> YGGGSSGGGS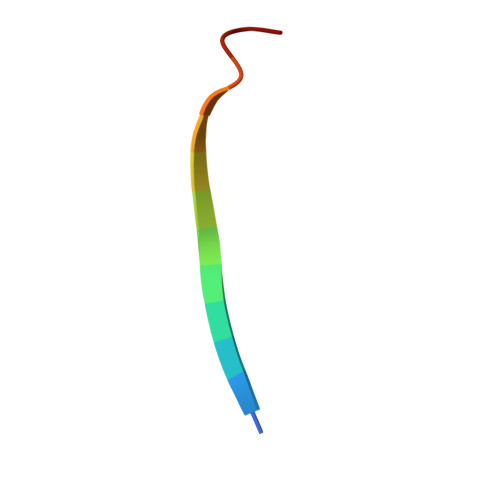SGGG>[2x]GPLGSEVIQALIFKDDGSLGLSISGGVGSSSFKSGDD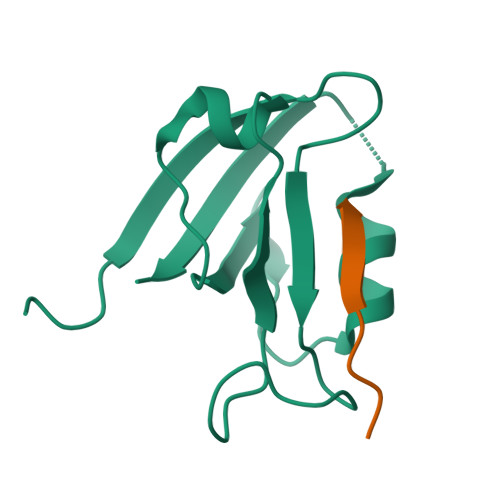GIFVSKIAKGGPCDNEGTLKIGDKILSVNEISFTGITHEKAVEILKNQDSKYMVVVERS;>[2x]NPNPETSV>[2x]MNAQTSTATQKHRVAPPPHVPGHLIREIDAYDLDGLEQGFHEAWKRVQQPDTPPLVWTPFTGGHWIATRGTLIDEIYRSPERFSSRVIWVPREAGEAYDMVPTKLDPPEHTPYRKAIDKGLNLAEIRKLEDQIRTIAVEIIEGFADRGHCEFGSEFSTVFPVRVFLALAGLPVEDATKLGLL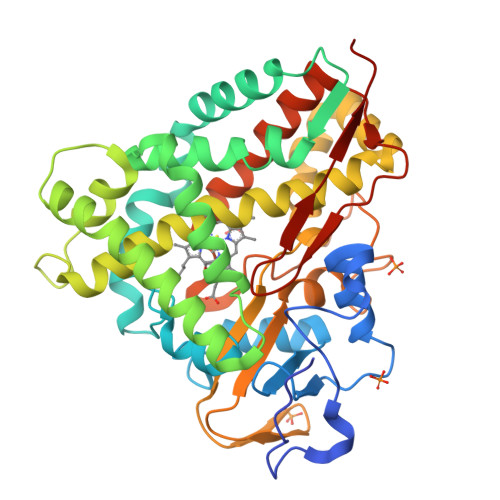ANEMTRPSGNTPEEQGRSLEAANKGFFEYVAPIIAARRGGSGTDLITRILNVEIDGKPMPDDRALGLVSLLLLGGLDTVVNFLGFMMIYLSRHPETVAEMRREPLKLQRGVEELFRRFAVVSDARYVVSDMEFHGTMLKEGDLILLPTALHGLDDRHHDDPMTVDLSRRDVTHSTFAQGPHRCAGMHLARLEVTVMLQEWLARIPEFRLKDRAVPIYHSGIVAAVENIPLEWEPQRVSA> MWSHPQFEKASTGREILEKLERREFTREVLKEALSINDRGFNEALFKLADEIRRKYVGDEVHIRAIIEFSNVCRKNCLYCGLRRDNKNLKRYRMTPEEIVERARLAVQFGAKTIVLQSGEDPYYMPDVISDIVKEIKKMGVAVTLSLGEWPREYYEKWKEAGADRYLLRHETANPVLHRKLRPDTSFE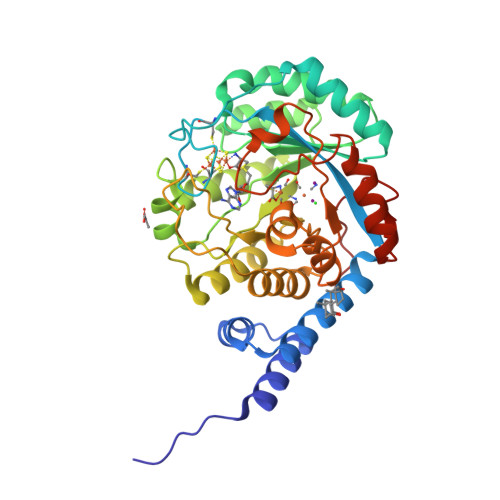NRLNCLLTLKELGYETGAGSMVGLPGQTIDDLVDDLLFLKEHDFDMVGIGPFIPHPDTPLANEKKGDFTLTLKMVALTRILLPDSNIPATTAMGTIVPGGREITLRCGANVIMPNWTPSPYRQLYQLYPGKISVFEKDTASIPSVMKMIELLGRKPGRDWGGRKRVFETV>MVDYSDCFEGISGGAIFYNTKNKEYNIYNKELIETRRSPASTFKIVSTLIGLEKGVINSKESVMGYDGTEYPNKNWNKNLSLEEAFKESCVWYYKKLIDKVDAKSVQNILDDLKYGNCDISEWEGDLKNGKGHLNGFWLESSLQISPKEQVQTMAKIFEGDTNFKKEHINILRDIMKIDVNDKNINVYGKTGTGFDEKNKRVDAWFVGML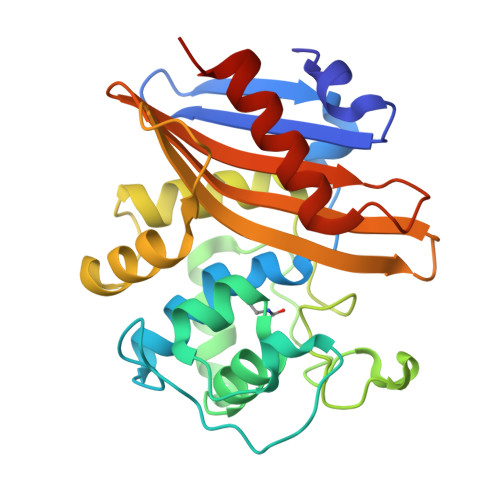EREGDTYYFAIKSDDSNKEITGPKVKEIAINIIKKYYSVREGAAL[4x]> MAKTLKDLQGWEIITTDEQGNIIDGGQKRLRRRGAKTEHYLKRSSDGIKLGRGDSVVMHNEAAGTYSVYMIQELRLNTLNNVVELWALTYLRWFEVNPLAHYRQFNPDANILNRPLNYYNKLFSETANKNELYLTAELAELQLFNFIRVANVMDGSKWEVLKGNVDPERDFTVRYICEPTGEKFVDINIEDVKAYIKKVEPREAQEYLKDLTLPSKKKEIKRGPQKKDKATQTAQISDAETRATDITDNEDGNEDESSDYESPSDIDVSEDMDSGEISADELEEEEDEEEDEDEEEKEARHTNSPRKRGRKIKLGKDDIDASVQPPPKKRGRKPKDPSKPRQMLLISSCRANNTPVIRKFTKKNVARAKKKYTPFSKRFKSIAAIPDLTSLPEFYGNSSELMASRFENKLKTTQKHQIVETIFSKVKKQLNSSYVKEEILKSANFQDYLPARENEFASIYLSAYSAIESDSATTIYVAGTPGVGKTLTVREVVKELLSSSAQREIPDFLYVEINGLKMVKPTDCYETLWNKVSGERLTWAASMESLEFYFKRVPKNKKKTIVVLLDELDAMVTKSQDIMYNFFNWTTYENAKLIVIAVANTMDLPERQLGNKITSRIGFTRIMFTGYTHEELKNIIDLRLKGLNDSFFYVDTKTGNAILIDAAGNDTTVKQTLPEDVRKVRLRMSADAIEIASRKVASVSGDARRALKVCKRAAEIAEKHYMAKHGYGYDGKTVIEDENEEQIYDDEDKDLIESNKAKDDNDDDDDNDGVQTVHITHVMKALNETLNSHVITFMTRLSFTAKLFIYALLNLMKKNGSQEQELGDIVDEIKLLIEVNGSNKFVMEIAKTLFQQGSDNISEQLRIISWDFVLNQLLDAGILFKQTMKNDRICCVKLNISVEEAKRAMNEDETLRNL;> MLNGEDFVEHNDILSSPAKSRNVTPKRVDPHGERQLRRIHSSKKNLLERISLVGNERKNTSPDPALKPKTPSKAPRKRGRPRKIQEELTDRIKKDEKDTISSKKKRKLDKDTSGNVNEESKTSNNKQVMEKTGIKEKREREKIQVATTTYEDNVTPQTDDNFVSNSPEPPEPATPSKKSLTTNHDFTSPLKQIIMNNLKEYKDSTSPGKLTLSRNFTPTPVPKNKKLYQTSETKSASSFLDTFEGYFDQRKIVRTNAKSRHTMSMAPDVTREEFSLVSNFFNENFQKRPRQKLFEIQKKMFPQYWFELTQGFSLLFYGVGSKRNFLEEFAIDYLSPKIAYSQLAYENELQQNKPVNSIPCLILNGYNPSCNYRDVFKEITDLLVPAELTRSETKYWGNHVILQIQKMIDFYKNQPLDIKLILVVHNLDGPSIRKNTFQTMLSFLSVIRQIAIVASTDHIYAPLLWDNMKAQNYNFVFHDISNFEPSTVESTFQDVMKMGKSDTSSGAEGAKYVLQSLTVNSKKMYKLLIETQMQNMGNLSANTGPKRGTQRTGVELKLFNHLCAADFIASNEIALRSMLREFIEHKMANITKNNSGMEIIWVPYTYAELEKLLKTVLNTL;> MSDLNQSKKMNVSEFADAQRSHYTVYPSLPQSNKNDKHIPFVKLLSGKESEVNVEKRWELYHQLHSHFHDQVDHIIDNIEADLKAEISDLLYSETTQKRRCFNTIFLLGSDSTTKIELKDESSRYNVLIELTPKESPNVRMMLRRSMYKLYSAADAEEHPTIKYEDINDEDGDFTEQNNDVSYDLSLVENFKRLFGKDLAMVFNFKDVDSINFNTLDNFIILLKSAFKYDHVKISLIFNINTNLSNIEKNLRQSTIRLLKRNYHKLDVSSNKGFKYGNQIFQSFLDTVDGKLNLSDRFVEFILSKMANNTNHNLQLLTKMLDYSLMSYFFQNAFSVFIDPVNVDFLNDDYLKILSRCPTFMFFVEGLIKQHAPADEILSLLTNKNRGLEEFFVEFLVRENPINGHAKFVARFLEEELNITNFNLIELYHNLLIGKLDSYLDRWSACKEYKDRLHFEPIDTIFQELFTLDNRSGLLTQSIFPSYKSNIEDNLLSWEQVLPSLDKENYDTLSGDLDKIMAPVLGQLFKLYREANMTINIYDFYIAFRETLPKEEILNFIRKDPSNTKLLELAETPDAFDKVALILFMQAIFAFENMGLIKFQSTKSYDLVEKCVWRGI;> MTISEARLSPQVNLLPIKRHSNEEVEETAAILKKRTIDNEKCKDSDPGFGSLQRRLLQQLYGTLPTDEKIIFTYLQDCQQEIDRIIKQSIIQKESHSVILVGPRQSYKTYLLDYELSLLQQSYKEQFITIRLNGFIHSEQTAINGIATQLEQQLQKIHGSEEKIDDTSLETISSGSLTEVFEKILLLLDSTTKTRNEDSGEVDRESITKITVVFIFDEIDTFAGPVRQTLLYNLFDMVEHSRVPVCIFGCTTKLNILEYLEKRVKSRFSQRVIYMPQIQNLDDMVDAVRNLLTVRSEISPWVSQWNETLEKELSDPRSNLNRHIRMNFETFRSLPTLKNSIIPLVATSKNFGSLCTAIKSCSFLDIYNKNQLSNNLTGRLQSLSDLELAILISAARVALRAKDGSFNFNLAYAEYEKMIKAINSRIPTVAPTTNVGTGQSTFSIDNTIKLWLKKDVKNVWENLVQLDFFTEKSAVGLRDNATAAFYASNYQFQGTMIPFDLRSYQMQIILQELRRIIPKSNMYYSWTQL;> MNVTTPEVAFREYQTNCLASYISADPDITPSNLILQGYSGTGKTYTLKKYFNANPNLHAVWLEPVELVSWKPLLQAIARTVQYKLKTLYPNIPTTDYDPLQVEEPFLLVKTLHNIFVQYESLQEKTCLFLILDGFDSLQDLDAALFNKYIKLNELLPKDSKINIKFIYTMLETSFLQRYSTHCIPTVMFPRYNVDEVSTILVMSRCGELMEDSCLRKRIIEEQITDCTDDQFQNVAANFIHLIVQAFHSYTGNDIFALNDLIDFKWPKYVSRITKENIFEPLALYKSAIKLFLSTDDNLSENGQGESAITTNRDDLENSQTYDLSIISKYLLIASYICSYLEPRYDASIFSRKTRIIQGRAAYGRRKKKEVNPRYLQPSLFAIERLLAIFQAIFPIQGKAESGSLSALREESLMKANIEVFQNLSELHTLKLIATTMNKNIDYLSPKVRWKVNVPWEIIKEISESVHFNISDYFSDIHE;> MSMQQVQHCVAEVLRLDPQEKPDWSSGYLKKLTNATSILYNTSLNKVMLKQDEEVARCHICAYIASQKMNEKHMPDLCYYIDSIPLEPKKAKHLMNLFRQSLSNSSPMKQFAWTPSPKKNKRSPVKNGGRFTSSDPKELRNQLFGTPTKVRKSQNNDSFVIPELPPMQTNESPSITRRKLAFEEDEDEDEEEPGNDGLSLKSHSNKSITGTRNVDSDEYENHESDPTSEEEPLGVQESRSGRTKQNKAVGKPQSELKTAKALRKRGRIPNSLLVKKYCKMTTEEIIRLCNDFELP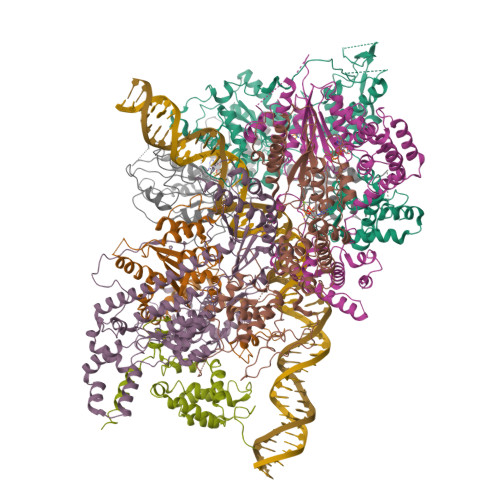REVAYKIVDEYNINASRLVCPWQLVCGLVLNCTFIVFNERRRKDPRIDHFIVSKMCSLMLTSKVDDVIECVKLVKELIIGEKWFRDLQIRYDDFDGIRYDEIIFRKLGSMLQTTNILVTDDQYNIWKKRIEMDLALTEPL;> MSAIPITPTKRIRRNLFDDAPATPPRPLKRKKLQFTDVTPESSPEKLQFGSQSIFLRTKALLQKSSELVNLNSSDGALPARTAEYEQVMNFLAKAISEHRSDSLYITGPPGTGKTAQLDMIIRQKFQSLPLSLSTPRSKDVLRHTNPNLQNLSWFELPDGRLESVAVTSINCISLGEPSSIFQKIFDSFQDLNGPTLQIKNMQHLQKFLEPYHKKTTFVVVLDEMDRLLHANTSETQSVRTILELFLLAKLPTVSFVLIGMANSLDMKDRFLSRLNLDRGLLPQTIVFQPYTAEQMYEIVIQKMSSLPTIIFQPMAIKFAAKKCAGNTGDLRKLFDVLRGSIEIYELEKRFLLSPTRGSLNSAQVPLTPTTSPVKKSYPEPQGKIGLNYIAKVFSKFVNNNSTRTRIAKLNIQQKLILCTIIQSLKLNSDATIDESFDHYIKAITKTDTLAPLQRNEFLEICTILETCGLVSIKKTKCKGKTKRFVDKIDVDLDMREFYDEMTKISILKPFLH> STTDQPLAKDKVALLIGNMNYREHPKLKAPLVDVYELTNLLRQLDFKVVSLLDLTEYEMRNAVDEFLLLLDKGVYGLLYYAGHGYENFGNSFMVPVDAPNPYRSENCLCVQNILKLMQEKETGLNVFLLDMCRKRNDYDDTIPILDALKVTANIVFGYATCQGAEAFEIQHSGLANGIFMKFLKDRLLEDKKITVLLDEVAEDMGKCHLTKGKQALEIRSSLSEKRALTDPIQGTEYSAESLVRNLQWAKAHELPESMCLKFDCGVQIQLGFAAEFSNV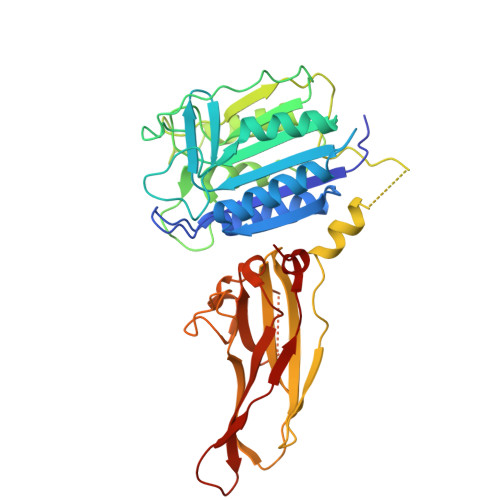MIIYTSIVYKPPEIIMCDAYVTDFPLDLDIDPKDANKGTPEETGSYLVSKDLPKHCLYTRLSSLQKLKEHLVFTVCLSYQYSGLEDTVEDKQEVNVGKPLIAKLDMHR>GSHMEFQRVHQQLLQSHHLFEPLSPVQLQELLASSDLVNLDKGAYVFRQGEPAHAFYYLISGCVKIYRLTPEGQEKILEVTNERNTFAEAMMFM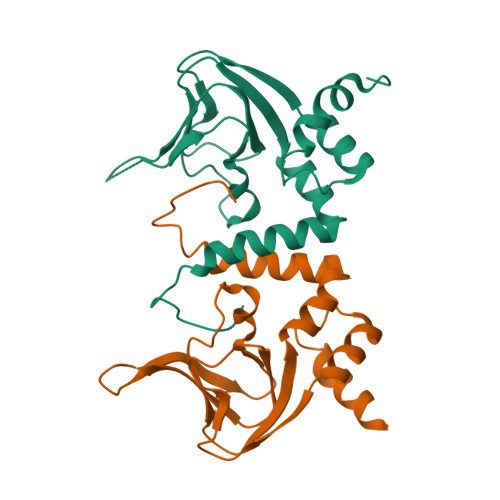DTPNYVATAQAVVPSQLFRFSNKAYLRQLQDNTPLALALLAKLSTRLHQRIDEIETLSLK[3x]> MGSAGKAAEERGLPKGATPQDTSGLQDRLFSSESDNSLYFTYSGQPNTLEVRDLNYQVDLASQVPWFEQLAQFKMPWTSPSCQNSCELGIQNLSFKVRSGQMLAIIGSSGCGRASLLDVITGRGHGGKIKSGQIWINGQPSSPQLVRKCVAHVRQHNQLLPNLTVRETLAFIAQMRLPRTFSQAQRDKRVEDVIAELRLRQCADTRVGNMYVRGLSGGERRRVSIGVQLLWNPGILILDEPTSGLDSFTAHNLVKTLSRLAKGNRLVLISLHQPRSDIFRLFDLVLLMTSGTPIYLGAAQHMVQYFTAIGYPCPRYSNPADFYVDLTSIDRRSREQELATREKAQSLAALFLEKVRDLDDFLWKAETKDLDEDTCVESSVTPLDTNCLPSPTKMPGAVQQFTTLIRRQISNDFRDLPTLLIHGAEACLMSMTIGFLYFGHGSIQLSFMDTAALLFMIGALIPFNV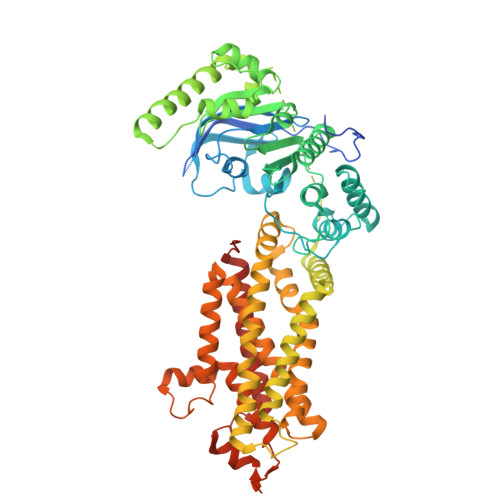ILDVISKCYSERAMLYYELEDGLYTTGPYFFAKILGELPEHCAYIIIYGMPTYWLANLRPGLQPFLLHFLLVWLVVFCCRIMALAAAALLPTFHMASFFSNALYNSFYLAGGFMINLSSLWTVPAWISKVSFLRWCFEGLMKIQFSRRTYKMPLGNLTIAVSGDKILSVMELDSYPLYAIYLIVIGLSGGFMVLYYVSLRFIKQKPSQDWASNSLEVLFQME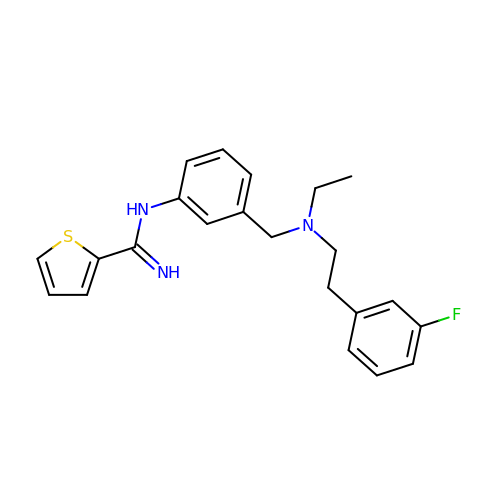N-[3-({ethyl[2-(3-fluorophenyl)ethyl]amino}methyl)phenyl]thiophene-2-carboximidamide | C22 H24 F N3 S | DFFRHUPAEPPGQC-UHFFFAOYSA-N> MSGSHHHHHHSSGIEGRGRLIKHMTAEAGITGTWYNQL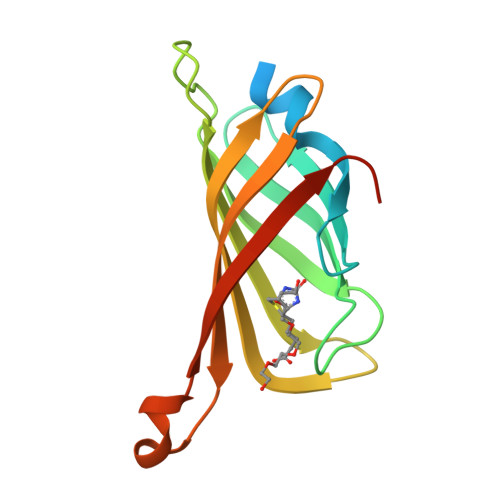GSTLIVTAGADGALTGTYESAVGNAEGSYVLTGRYDSAPATDGSGTALGWTVAWKNNYRNAHSASTWSGQYVGGAEARINTQVLTTSGTTEANAWKSTLVGHDTFTKVKPSAASI>MDNQHKKIKGYRDLSQEEIDMMNRVKELGSQFEKLIQDVSDHLRGQYNASLHNRDEITRIANAEPGR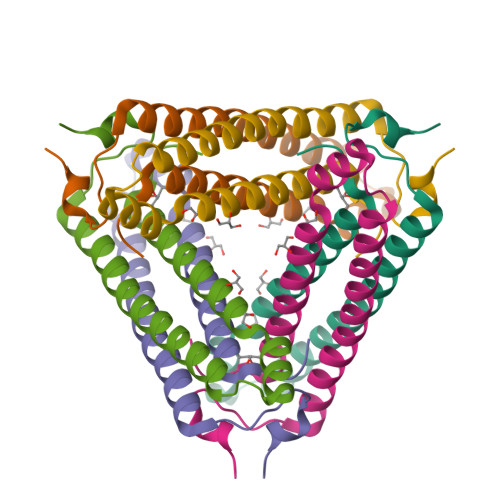WLAIGKTDIQTGMMAIIRAIAQPDSF[6x]>MSIDKSYCGFIAIVGRPNVGKSTLLNKLLGQKISITSRKAQTTRHRIVGIHTEGAYQAIYVDTPGLHMEEKRAINRLMN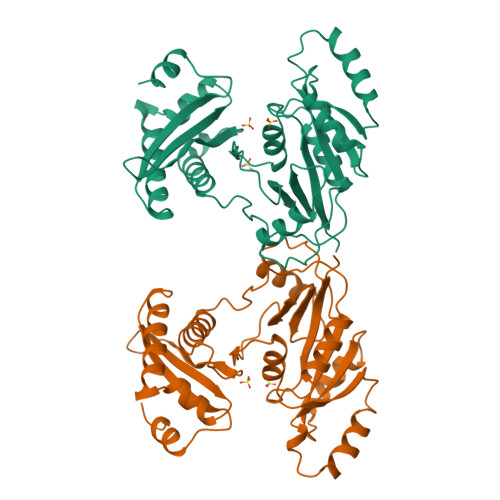KAASSSIGDVELVIFVVEGTRWTPDDEMVLNKLREGKAPVILAVNKVDNVQEKADLLPHLQFLASQMNFLDIVPISAETGLNVDTIAAIVRKHLPEATHHFPEDYITDRSQRFMASEIIREKLMRFLGAELPYSVTVEIERFVSNERGGYDINGLILVEREGQKKMVIGNKGAKIKTIGIEARKDMQEMFEAPVHLELWVKVKSGWADDERALRSLGYVDDL[2x]> XXXXXEDMGRLHLDDGKSPNHGEIAKVGEGKYREDFQM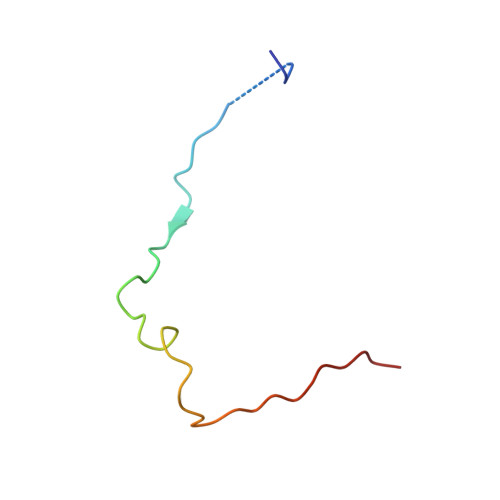DEGE>MRARLYAAFRQVGEDLFAQGLISATAGNFSVRTKGGFLITKSGVQKARLTPEDLLEVPLEGPIPEGASVESVVHREVYRRTGARALVHAHPRVAVALSFHLSRLRPLDLEGQHYLKEVPVLAPKTVSATEEAALSVAEALREHRACLLRGHGAFAVGLKEAPEEALLEAYGLMTTLEESAQILLYHRLWQGAGPALGGGE[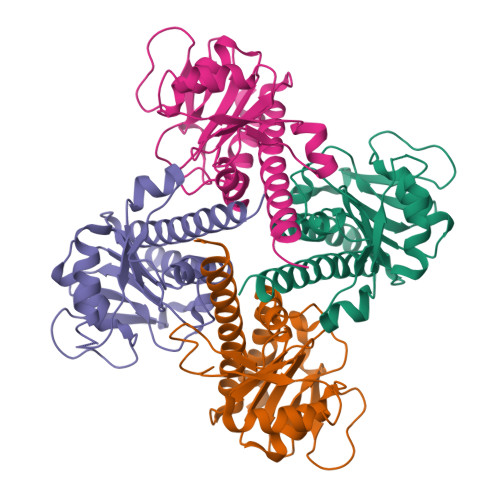8x]>GIEDLIDTAIKNALRVSQPPSTQSTEATSGVNSQEVPALTAVETGASGQAIPSDVVETRHVVNYKTRSESCLESFFGRAACVTILSLTNSSKSGEEKKHFNIWNITYTDTVQLRRKLEFFTYSRFDLEMTFVFTENYPSTASGEVRNQVYQIMYIPPGAPRPSSWDDYTWQSSSNPSIFYMYGNAPPRMSIPYVGIANAYSHFYDGFARVPLEGENTDAGDTFYGLVSINDFGVLAVRAVNRSNPHTIHTSVRVYMKPKHIRCWCPRPPRAVLYRGEGVDMISSAILPLAKVDSITTF[5x];>[5x]SPNVEACGYSDRVRQITLGNSTITTQEAANAIVAYGEWPTYINDSEANPVDAPTEPDVSSNRFYTLESVSWKTTSRGWWWKLPDCLKDMGMFGQNMYYHYLGRSGYTIHVQCNASKFHQGALGVFLIPEFVMACNTESKTSYVSYINANPGERGGEFTNTYNPSNTDASEGRKFAALDYLLGSGVLAGNAFVYPHQIINLRTNNSATIVVPYVNSLVIDCMAKHNNWGIVILPLAPLAFAATSSPQVPITVTIAPMCTEFNGLRNITVPVHQ;>[5x]GLPTMNTPGSNQFLTSDDFQSPCALPNFDVTPPIHIPGEVKNMMELAEIDTLIPMNAVDGKVNTMEMYQIPLNDNLSKAPIFCLSLSPASDKRLSHTMLGEILNYYTHWTGSIRFTFLFCGSMMATGKLLLSYSPPGAKPPTNRKDAMLGTHIIWDLGLQSSCSMVAPWISNTVYRRCARDDFTEGGFITCFYQTRIVVPASTPTSMFMLGFVSACPDFSVRLLRDTPHISQSKLIGRTQ;>[5x]MGAQVSTQKTGAHENQNVAANGSTINYTTINYYKDSASNSATRQDLSQDPSKFTEPVKDLMLKTAPALN

Non-polio enteroviruses (NPEVs) from the family of Picornaviridae are nonenveloped viruses composed of (+) ssRNA genomes that infect humans and cause a variety of human diseases. For this proof-of-concept study, we selected CV-A21 viral strain responsible for a substantial proportion of enterovirus-associated acute respiratory tract infections in humans. Herein, we introduce an EMPEM pipeline for rapid structural analysis of pAb responses elicited by enteroviruses using whole viral particles. Using a combination of nsEM- and cryoEM-based polyclonal epitope mapping, we identified two primary immunogenic sites on the surface of CV-A21 located near the 3-fold and 5-fold axes.

Through iterative rounds of focused classification, we reconstructed maps featuring structurally distinct polyclonal antibodies bound to epitopes at near-atomic resolution (structurally distinct polyclonal antibody class—pAbC). We resolved two distinct polyclonal antibodies targeting Site-1 and three against Site-2. We next relaxed atomic models into the pAbC1-1, pAbC2-1, and pAbC2-3 cryoEMPEM maps. Given the polyclonal nature of bound antibodies and the inherent lack of sequence information, the variable Fab domains (Fv) were represented as poly-Alanine models. Specific epitope contacts and angle of approach were highly similar for Site-1 antibodies while Site-2 pAbs displayed greater diversity; consistent with nsEM analysis. Site-2 is particularly interesting because it is in immediate proximity to the receptor binding site (RBS) for CV-A21. While antibodies targeting Site-1 are distal from the RBS and it is unlikely that they would interfere with receptor binding as Fabs, antibodies against Site-2 sterically block ICAM-1 from accessing the RBS and may be able to suppress viral entry. Site-2 pAbs display high similarity in epitope and angle of approach to 1D5 mAb, and a partial overlap with 18A7 mAb that binds directly on top of the 5-fold symmetry axis. Importantly, all pAbs bind in a manner that does not block the accessibility to the symmetry-related neighboring binding site. While both Site-1 and Site-2 are highly immunogenic, the sequence conservation is relatively low, and elicited antibody responses are unlikely to cross-react with other strains of CV.>SNAMKTLFLQYPACSTCQKAKKWLIENNIEYTNRLIVDDNPTVEELKAWIPLSGLPVKKFFNTSGVVYKELKLSSKLPTMTEEEQIALLATNGKL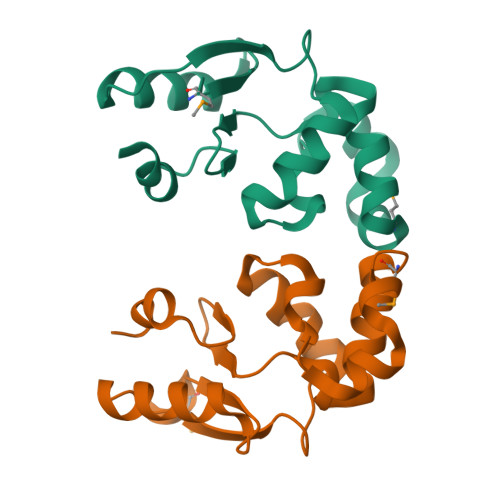VKRPLVVTERFVLVGFKPEEWEKLK[2x]In this study, the structure, biological properties, and vaccine potential of the Ng-adhesin complex protein (Ng-ACP) are presented. Ng-ACP is structurally homologous to Neisseria meningitidis ACP and MliC/PliC lysozyme inhibitors. Ng-ACP functions as a human lysozyme inhibitor. Thus, in summary, Ng-ACP is a stable, highly conserved protein that functions principally as a lysozyme inhibitor.

The crystal structure of recombinant Ng-ACP (rNg-ACP) protein was solved at 1.65 Å. A second expression construct that lacked the N-terminal signal peptide sequence and instead contained a C-terminal 6×His tag had a predicted length of 111 amino acids with a Mr of 12,372.05. The latter construct was used to purify rNg-ACP by Ni-NTA affinity chromatography and size exclusion chromatography (SEC) in soluble form for crystallization and structure determination and also immunogenicity studies. The overall fold of rNg-ACP was an eight-stranded β-barrel, and the structure was comprised of two sets of four stranded antiparallel β-sheets (β1 to β4 and β5 to β8), with the disulfide bridge between Cys37 and Cys120 stabilizing the interaction between β8 and β1. Ng-ACP was superposed with Nm-ACP and with members of the MliC/PliC family lysozyme inhibitors found in other Gram-negative bacteria, e.g., Salmonella Typhimurium (St-PliC) and Brucella abortus (PliC). The superposition of Ng-ACP and the Brucella abortus PliC-lysozyme complex showed a conformation of “loop 4” incompatible with lysozyme binding; furthermore, helix α1 of Ng-ACP would also clash with lysozyme. We investigated this further and provide a conservation analysis that is based on sequence alignment of ACP proteins from different Neisseria species. Interestingly, there is little conservation in the region around β6, suggesting that this region is not involved in formation of a conserved interface (compare the green region in Fig. 3). While our analysis revealed some conservation in loop 4, this loop was much shorter in the MliC/PliC family of proteins, explaining why the loop clashed with lysozyme in the superposition. However, the analysis also reveals conservation in the loop 4 region, which is involved in lysozyme recognition, and hence interaction might occur through this region using a different binding mode; this would explain the difference in sequence length in this region between Ng-ACP and PliC proteins.

> AGTDNPTVAKKTVSYVCQQGKKVKVTYGFNKQGLTTYASAVINGKRVQMPINLDKSDNMDTFYGKEGGYVLSTGAMDSKSYRKQPIMITAPDNQIVFKDCSPRLEHHHHHH>[3x]MRRFGSKFASGLASRCALACPLASAATAPAGASTTSSTSSAQKSFFKTTEMIGYVHSIDGTIATLIPAPGNPGVAYNTIIQIQVSPTTFAAGLVFNLEKDGRIGIILMDNITEVQSGQKVMATGQLLHIPVGAGVLGKVVNPLGHEVPVGLVTRSRRLLDSTLGKVDTGAPNIVSRSPVNYNLLTGFKAVDTMIPIGRGQRELIVGDRQTGKTSIAVSTIINQVRINQQILSKNAVISIYVSIGQRCSNVARIHRLLQSYGALRYTTVMAATAAEPAGLQYLAPYAGVTMGEYFMNRGRHCLCVYDDLSKQAVAYRQISLLLRRPPGREAYPGDVFYLHSRLLERAAMLSPGKGGGSVTALPIVETLSNDVTAYIVTNVISITDGQIYLDTKLFTGGQRPAVNIGLSVSRVGSSAQNAAMKGVAGKLKGILAEYRKLAADSVGGQQVQTIPMIRGARFVALFNQKQPSYFMNAIVSLYACLNGYLDDVKVQYVKFYEYLLVHRDLGIMYGTAKNKFFYMYVQELNYLIRFFTLNSPILHGELEEMLKQHTHLFLQHYQSKMNAIKSEKDVKALKNLLYSCKRAV;>[3x]MLTRFRSAVLRGAVSITGARAASTAPVADHKGRVGHVSQVIGAVVDVHFADGVPPVLTALDVVDKLGRDEPLTLEIVQHLDAHTGRCIAMQTTDLLKLKAKVVSTGGNISVPVGRETLGRIFNVLGDAIDQRGPVGEKLRMPIHAVAPKLADQAAEDAVLTTGIKVIDLILPYCKGGKIGLFGGAGVGKTVIIMELINNVAKGHGGFSVFAGVGERTREGTDLYLEMMQSKVIDLKGESKCVLVYGQMNEPPGARARVAQSALTMAEYFRDVEGQDVLLFIDNIFRFTQANSEVSALLGRIPAAVGYQPTLAEDLGQLQERITSTTKGSITSVQAVYVPADDITDPAPATTFSHLDATTVLDRAVAESGIYPAVNPLECASRIMDPDVISVDHYNVAQDVVQMLTKYRELQDIIAVLGIDELSEEDKLIVDRARKLVKFLSQPFQVAEVFTGMTGHYVQLDDTIDSFSGLLMGTYDQVPEMAFYMVGGINSVLEKAKKMAEEAAELEKMRRARVAQASS;> MSGKLRLYKEKLEGYNRFYSIVKTIKMVTLAKYRAAQGRIRTRDFSLRYTELAFSKPQASRDAVVAAKNALVYIPITTNRGSCGALNSNIVRCIDSVVSSKMVLMPVGKRGIDSFSKLYPDEFRYGIINDMKESMHFGYATFVIENAYEVSKDADRYQVIFNRFVSAGVQRNAVYNIPSYEKWKEDLADAASSDNQKNRYLFANALQNEEEQLIRDFFDFHAALAVLNAVGENELSEQAARLVAVEGQLTNISSLQQRTSSLYNKTRQFGITAALIEILSAMSSLEGNAMKGVRRNKFWEGAVTK;> MFRTFGRRLVSCTLPLLQSAPHDLPEGFEFMEHKVVNKDIHAPHENLETLRLTLTRQDEFLLREEPVKCVTVTGTNGEYGIYPGHAYKIVQLNPSPLTVEYTDGTTKKYFVSGGFAHINNEGSCDVNTVECTLLDDLDLAIAEKELAAQQAALGSAKDDKAKSVVEIRISVIEAVIAALKHH;> MIRRSCALLSSSWRDHGISYLKYLNVCTETLHSTVKESRRAKYERWSKPCYTAQRPDGAGGQETIDKVPIHTKDY;>[3x]MMRRVYSPVFCSVAAARFAATSAAKKYDLFGYEVDTNTAPWIEKIKKCKYYDEAGEVLVNMNVSNCPPDIATYNATLQCIYQSPSKQSTPVDNESKFCAMMDLLEEMQHRNRLKPNEESWTWVMKECVKSGQFRLGYCIQQVMETECKGCPADLVKANEANAQKAKTEGKEHPGHLSQQAGLFDVKVE;>MSAKAAPKTLHQVRNVAYFFAAWLGVQKGYIEKSANDRLWVEHQRKVRQQNVERQQALDSIKLMQQGVRATTPGQLEGVPAELQQLAEAFTK[2x];>[2x]MSSTKCAVACKIMTPLCNAASKVQARSAKKLAALTDAGIQKTISEHNANGTDAAVSSTKRYLAEQRQLFHYRVVRFFDECHYIISGEYFAQYTKVNLIWDLRFLTKLVVLFLIGTVLGRQSIFPPIDPDSPLVEALVTKVNPNY;> MFRRLSSSARAVVAARFYTPPEGLKKLYASDFENSKYPLNIVPSDSVLFAKFLYKAAEEKGNFDNILSDFQKIAAAASKLPIFWERTAVVEKIPEFKQLSEPTFFTLVWMQNNGMLELIQEVAEVYETFVNAKQKKAVAKIFVAPGGEKNVEEARRVAEELHKGLKELADYTLVLKTVVDRTIVKGFAVELAGQYVNKAEGQQKQAGRADEVDYTNLPAPKPQKTVWDDNIETEVLRKYLDGLSQYDMEEAKYGV;>MMRRLALQSSIRRATPFATPLVASTKALNPMCSAITIREASTVAISVQGLHYVGTGLAAIALAGVGLGIGTIFGNLLVACARQPNLTKMLFNYAILGFALTEAIGLFALMLAFLMLFS[10x];> MFLFFFCDLFWLRLLLCMYYCVWSRLCFIVYFNCLMLIFDFLLFCLFDLYLFVGLCLFLLLWFMLFNLYSLILYYCITYLNLYLLFCIVFLLYIAFLFLFCFLCDFFLFNNLLVGDSFMDVFFIRFLLCFLECFSLLCRCLSTFLRLFCNLLSSHFLLLMFFDFFYFIFVFFFYGVFCYWFILFIFVFCFCLLFYVFLYLLDLFAAILQLFIFCNMILQLIMDFLLFLLFV;> MLRRLGANVSNMARPMNKYAVTVSPRRHLEPMSTWYLASWAMVWYYAFFFWMPMVWTDIMVPSFVYNKLPVIHFLQEKRAEQKLRRVLDETYTEWTEELDQAHVTDAITRSLNI;> MRRVSSPNITIQSVRWISGVSPLLYFPPTTTSTTNREDQINKNTNIAIQMIKRYKGEVPPHYTRKSSATIEQVEKEIDALLGGAEKLRKTSTDDQPMDKLTLMERCLRHALWSYHKEEGRYDFDQIGRWVVYTPEDEVKLAQLKREVEAKEKLAALRKRREEEGLPGGPVPRINWPQEYSS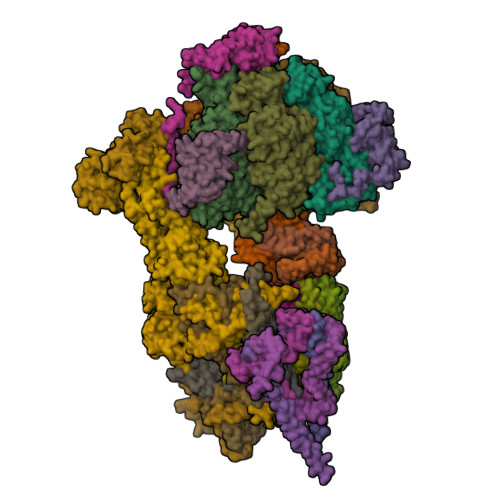FIDREPVVAKRIRYDTLASTTLERDEKQIESTLQQYRRASQDKRLDDLVDLLERFKPVLAREAIMQRLTIKHLEGQLGVWRYMDWCPEVRDRAELEVDITGWQWWSPLEERRLLPVRLRSVNEVREIMSKTQAKKSAEAAERNPIVTQTSTGDNARDRLLKEVLALQARINQRDEVEPSQTEQKKKAHH;> MQGSWSVLKKNCSNFFPGLLAFAQQTQEAYGIWLRIYNRQQKYGPTDFVEQSETFSPDYHKRFHSQDKNMWVDKELCTEVSQKEVARLMTYKLDMWRMAHCAGALLATGGYAIPFGLFWLANDTWVPSSFNLTGEELRAWREAQDLYRYRSAPSYLTDTKWHFDFHAYPWNETQERAWDDLFEKNDVRRDPKVVRPAAEMYDGFIKFELIRRKSLRHLCRSMNIPTFPMLARLCNGTRVRDYWNLAWCEDYMVITQRLHESMTDEELYDYAWRRYLAPYDKNLNREQLMERVEDYFEFLGPDFVAHGKAPNLVILTNYVLGYYNDPAYLEGDISELDKNDYDHLASWGKDAFLRRLEFENGPLRDQVEAHTQRLLAERAAIAKGDNAAAVEGRHTA;> MVLFSTYRSSRLVSKEFLHGPVMRFRALGEYYFQRAWNGTLNWALPGEYRLYAVMIPFIYFYHRWHNDHTLDRDHVEKAMIMRWGGTLEDVRKLSAKDQLRVRCFTDIEKLYSAYGPKDTYLQPPGDTLPGKDFYRKAGGAQAHH;> MSKQLTFISAGATAAVLQSASAIVSKVAGGRVQTKTAKEAGRHAVVVGPETPIGVHTAVTEVPKSAQDPLFSGVSTVVVRAVLPRAAPDSVQLRDALDVYASAGIDTKEEVRSATEAFKKSAEVAVGKAKAKGVKRIVLVVKQASKHNCINELFKKISTETIESAGLTTEVVGTAAVANQLIVNPESLGVVLLNDVAATEQIELAFAGVVGGVSRVYHTVEGGKISAGHSFKSVALAVAQELRELGLSSEADKVEAAASKNPRAVVSAL;> MRRTFISFSAASAAAAAPVTSTKMQTLHKLLTGEVSFKNKAPVKDCNIVHQFGENWATELSAYAKTLPAEQQKIIVRQIARVKLTRYTVAELAAYCGDGPALLDETARAANIEQGVAFVKAKGVEAFEKYVAEESTNANWKPEEAKKFIEDVKAKAK;> MVYTRWKCDRLPVFQLKLFTQEYPMHAAVGIFTIIFLWKHMSHCSEETERKYGWWAGYPYWRDPIARRNETKYKQMIINNDVDITHPKWTGCSVEQLEELSRVV;> MTKYELKMQYFDEWMIRWRKFQTESDWEIEKGRQWWRRFNMAVSGALFCGLVLYTSGTATLKRQYGLPHFFDIGVDGQAKETMLKTLTSRWRYTPQGYGRVLITGVPTYILFVTLEHYRERRRMQQYLQQNTVFGEQMRRLLSTGKIEEYLPVNIKATLPASQQAIYNY;> MLRRSSAALIRRTPVRHSGGELFVRPKLEEIPPADQCRGFFGPLNDSLKFLRLLDIKWMMNRAVAMRREYLIATPTLFTFIWMFTWKGAVIYFWGDRAPPRRMDWNTEETGRLPLGFKPTPAPL;> MLRKTPLFAMATTRKALVGNGPTFSTGGECMNTCDIQNAFPMNDRGVRSSSPFQEPNTAIYDSYLAWTYFQPMDVHIEKLPAPEAKYYQRHTKKPWDVSSTELTEIQSRKKYFQTLGYLVAFIYLYFLMPKEKSFSGLSGPDGHWIMLPKGRPELF;> MSSGFHFHDVSNDAIKGMPPSEALHKHLENAQLAHRICLAKALKAGEPPVEKCALTWGEVLIRYQAWSEYRPPFQDSVAQAKYKKYWSKKRQEEDDKNPFK;> MLRRLVPRVMMAPMGGATALCTSRGYNMLVFRDPKRRPQLSEEERAKVVVNQAEWPEEFKDFDPDDPYKNSPEIIKGMSSWNLFLWGVECAFIYQFYELVFPKSI;> MTENIEAVMSDFWSNPADHFRPNLKALTLYAERQHYVDRWLHVKERWLAPWYLPWWSPLFQLGTWYSQRSRNLFLVENHLSYRPYKFRRNDEDRNNPY;> MLLGGFVPRRFSQFNRDPCWMFFIFSVGFWLGEYPAMMIKYNARDLVYDPHRYVWSHHDDHH>MNMDVIKSFTEQMQGFAAPLTRYNQLLASNIEQLTRLQLASANAYAELGLNQLQAVSKVQDTQSLAALGTVQLETASQLSRQMLDDIQKLSALGQQFKEELDVLTADGIKKSTGKA[16x]

PHAs are stored intracellularly as granules surrounded by a layer of phospholipids and several types of granule-associated proteins including PHA synthases, PHA depolymerases and a group of proteins known as phasins or PhaPs. PhaPs are proteins that bind to the surface of PHA granules, and can be regarded as an interphase between the cytoplasm and the hydrophobic PHA granules which functions in preventing granular coalescence. In this study, the crystal structure of PhaPAh has been revealed, and a mechanism proposed for its binding to hydrophobic PHA materials. Generally speaking, PhaPAh forms tetramers with 8 α-helixes in aqueous solution and two different types of peptide chains were observed in these tetramers, whereby a hydrophobic and a hydrophilic surface is present in each monomer.

PhaPAh native crystals diffracted to 3.0 Å, as observed using the Shanghai Synchrotron Research Facility (SSRF) BL17U beamline. After rounds of phase improvement and extension, model building, and refinement, the final structure was refined to a resolution of 3.00 Å with Rwork of 22.70% and Rfree of 29.50%. Size-exclusion chromatography and dynamic light scattering (DLS) analyses indicated that PhaPAh exists as a tetramer in solution and the final model in the asymmetric unit consists of four PhaPAh tetramers accordingly. The overall shape of the tetramer somewhat resembles a flat rectangular brick, with two short N-terminal helices from chains A and D protruding outwards from two opposite sides of the “brick”. The four monomers in the PhaPAh tetramer adopt two distinct conformations: type I, observed in chains A and D and type II, observed in chains B and C. When chains A and C are superimposed based on helix 2, a major conformational difference is found between types I and II, in which the position of the entire helix 3 shifts downwards in chain C. A very significant phenomenon, observed in both conformations, was the focused distribution of hydrophilic and hydrophobic residues on two opposite sides of the PhaPAh monomer. The formation of the tetramer can accordingly be rationalized the following way: chains A and D expose their respective hydrophobic surfaces to each other, while loop regions of these two chains are next to each other forming a shape resembling chopsticks. The still exposed hydrophobic regions of the stacked A–D dimer then recruit chains B and C through hydrophobic interactions to form the tetramer. The recruitment of chains B and C leaves no hydrophobic region exposed to the solvent environment in the tetramer.NG,NG-DIMETHYL-L-ARGININE 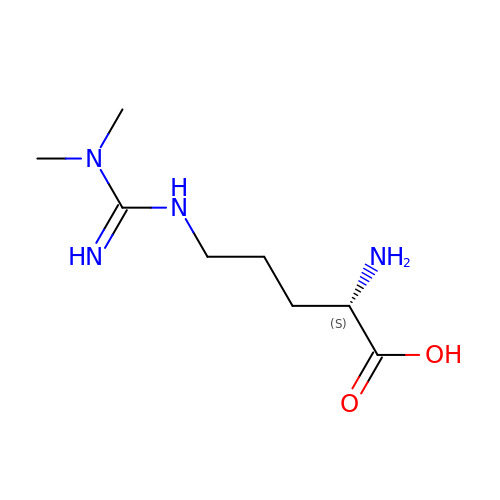| C8 H18 N4 O2 | YDGMGEXADBMOMJ-LURJTMIESA-N To address this challenge, we develop a computational “anchor extension” methodology for targeting protein interfaces by extending a peptide chain around a non-canonical amino acid residue anchor. To test our approach using a well characterized model system, we design cyclic peptides that inhibit histone deacetylases 2 and 6 (HDAC2 and HDAC6) with enhanced potency compared to the original anchor (IC50 values of 9.1 and 4.4 nM for the best binders compared to 5.4 and 0.6 µM for the anchor, respectively). SHA can coordinate to the zinc ion in the active site of HDACs. In all the crystal structures we obtained, the thiol functional group of SHA coordinates the catalytic Zn2+ ion with a Zn2+– S separation of 2.3 Å in a distorted tetrahedral geometry reminiscent of that observed for the inhibitor Largazole.

However, we obtained a crystal structure of des4.3.1 with zebrafish (Danio rerio) HDAC6 at 1.7 Å resolution. This peptide inhibits human HDAC6 with an IC50 value of 17.1 nM, 88-fold more potently than HDAC2. The binding orientation of the peptide is similar to the design model, but the structure of the peptide is very different. In particular, d-Arg8 occupies the negative phi region of the Ramachandran map (φ = 166° in the design and -46° in the crystal structure). If the d-Arg is replaced by l-Arg during conformational sampling, the lowest energy structures are very close to the crystal structure. The newly adopted conformation is complementary in shape to the contour of the active site and stabilized by several backbone-backbone hydrogen bonds and n → π* interactions. The peptide also forms both direct and water-mediated hydrogen bonding interactions with residues in the outer active site cleft of HDAC6. Notably Ser531 of HDAC6 donates a hydrogen bond to the carboxylate group of Asp7 and accepts a hydrogen bond from the backbone amide of SHA; Ser531 similarly accepts a hydrogen bond from the backbone amide of bound acetyl-lysine HDAC substrates. Mutation of Asp7 to Ala did not result in a significant change in IC50 for HDAC6 or HDAC2, while mutation of D-Arg8 → D-Ser raised the IC50 10-fold, suggesting an essential role for this residue, possibly due to its complementarity to the negative electrostatic surface potential of HDAC6 in this region. HDAC6 was not the target in the computational design calculations, and it is unclear whether the binding mode of the peptide to HDAC2 would be similar or different from that observed in the HDAC6 structure.

> SNAGGSSPITGLVYDQRMMLHHNMWDSHHPELPQRISRIFSRHEELRLLSRCHRIPARLATEEELALCHSSKHISIIKSSEHMKPRDLNRLGDEYNSIFISNESYTCALLAAGSCFNSAQAILTGQVRNAVAIVRPPGHHAEKDTACGFCFFNTAALTARYAQSITRESLRVLIVDWDVHHGNGTQHIFEEDDSVLYISLHRYEDGAFFPNSEDANYDKVGLGKGRGYNVNIPWNGGKMGDPEYMAAFHHLVMPIAREFAPELVLVSAGFDAARGDPLGGFQVTPEGYAHLTHQLMSLAAGRVLIILEGGYNLTSISESMSMCTSMLLGDSPPSLDHLTPLKTSATVSINNVLRAHAPFWSSLR;> ASDRXFLK> SMLQSNEYFSGKVKSIGFSSSSTGR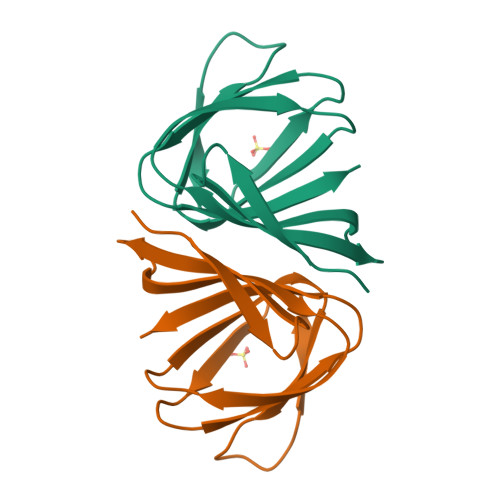ASVGVMVEGEYTFSTAEPEEMTVISGALNVLLPDATDWQVYEAGSVFNVPGHSEFHLQVAEPTSYLCRYL> ATYKVYPWGVNDPSKGSRSTVENPWNLAASEFTWLSDGSNNYTTTRGNNGIAQVNPSGGSTYLNNYRPDSPSLKFEYDYSTSTTTPTTYRDASIAQLFYTANKYHDLLYLLGFTEQAGNFQTNNNGQGGVGNDMVILNAQDGSGTNNANFATPADGQPGRMRMCLWTYSTPQRDCSFDAGVVIHEYTHGLSNRLTGGPANSGCLPGGESGGMGEGWGDFMATAIHIQSKDTRASNKVMGDWVYNNAAGIRAYPYSTSLTTNPYTYKSVNSLSGVHAIGTYWATVLYEVMWNL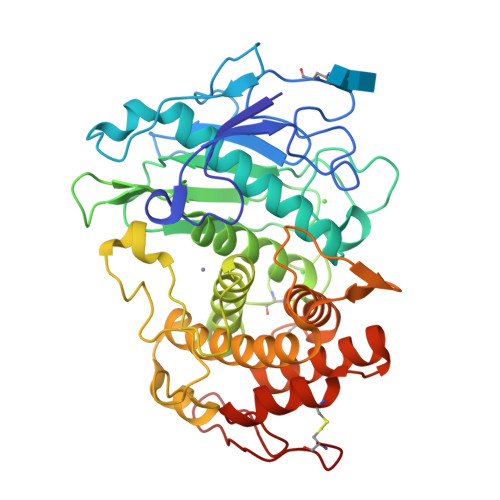IDKHGKNDADEPKFNNGVPTDGKYLAMKLVVDGMSLQPCNPNMVQARDAIIDADTALTKGANKCEIWKGFAKRGLGTGAKYSASSRTESFALPSGC[(4S,5R)-4,5-bis(4-chlorophenyl)-2,4,5-trimethyl-4,5-dihydro-1H-imidazol-1-yl]{4-[3-(methylsulfonyl)propyl]piperazin-1-yl}methanone | 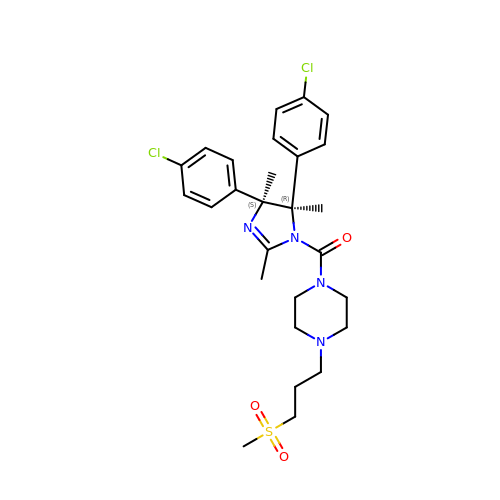C27 H34 Cl2 N4 O3 S | MCLBNCWBALNIBY-RRPNLBNLSA-N>SNAMSVEKQTAMRRTFAIISHPDAGKTTLTEKLLLFGGAIQLAGTIKSRKAARHATSDWMELEKQRGISVTTSVMQFPYKDYLINLLDTPGHADFTEDTYRTLTAVDSALMVIDAAKGVEPRTIKLMEVCRLRHTPIMTFINKMDRDTRPSIELLDEIESILRIHCAPVTWPIGMGKYFKGIYHLIEDAIYLYQPGKHERVGESERIEGINNPELDKKLGDLASELRNEIELVKGASHPFEREGYLKGELTPIFFGSAINNFGVGELLDAFVKEAPPPQGRETNSRLVKPEEEKFSGFVFKIQANMDPGHRDRIAFLRIASGQYQKGMKAYHVRLKKEIQINNALTFMAGKRENAEEAWPGDIIGLHNHGTIQIGDTFTQGERFKFTGIPNFASELFRLVRLKDPLKQKALLKGLTQLSEEGATQLFRPLDSNELILGAVG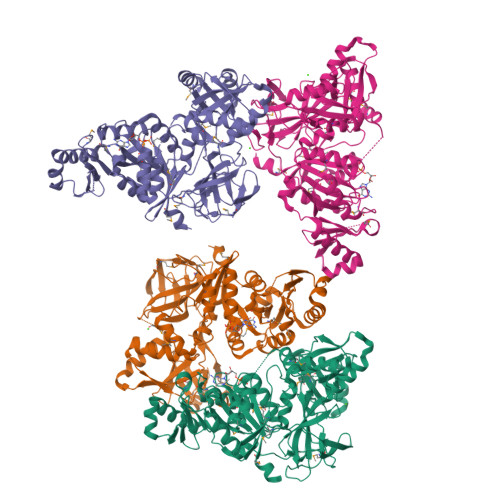LLQFDVVAYRLENEYNVKCVYESVNVVTARWVICDDKAVLERFNQEQSRNLAYDGGGHLTYLAPSRVNLEITMEKWPEIQFSETREH[4x]>[2x]MTDSEEYHLPQHVAIIMDGNNRFAKKNQMQKGDGHREGKNVLDPIVEHCVKTGVRALTVFAFSSENWNRPQYEVDLLMKLLEETIHEQIPRMKKFNIALRFIGDRSRLPSHLVALMEDAEQQTAHHEAMTLTIAVSYG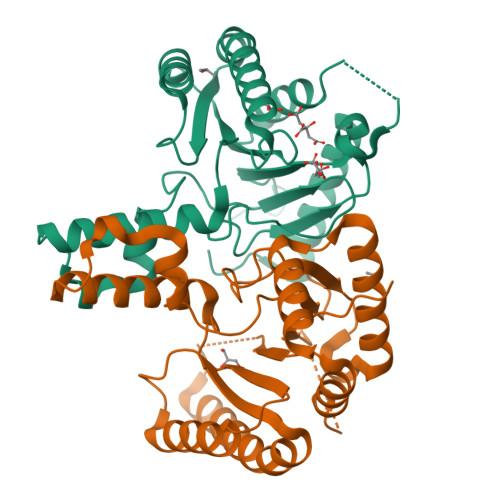GMWDIANAAKQVAQAVSRGEIDADQINVDLFAKYVSLNDLPAVDLLIRTGGDFRISNFLLWQAAYAELYFTDTLWPEFTVEEFDHALNVFSGRERRFGKTSEQIQQEKIEKLLEHHHHHH methyl 6-[4-[[N-[2-[(2R,3S,4R,5R)-5-(6-aminopurin-9-yl)-3,4-bis(oxidanyl)oxolan-2-yl]ethyl]carbamimidoyl]amino]butylcarbamoylamino]-4-oxidanyl-naphthalene-2-carboxylate | C29 H36 N10 O7 | 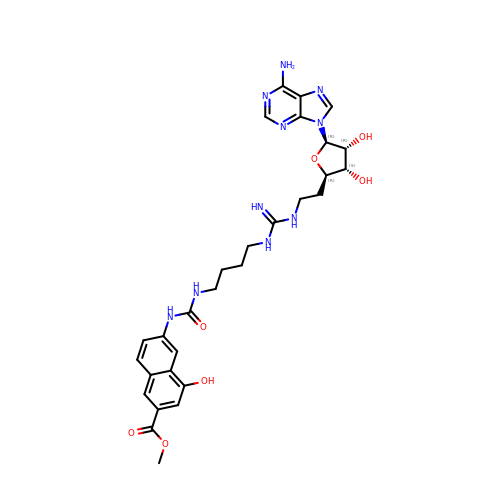QVOKJKWHZRTVQQ-HUBRGWSESA-N>[2x]MSAQLRAAAAITPAARRVISGPAAVRRFHHYHHLPTGGIQRVEIAARGLRRSVQFPALANAYHNNAVIVRNASFTRLLPKLALKFIRVPALFGGMMLGAVGWVQYQAIKVSNSAQEFYGNIKATVADTAFSVWSSAVDIAEQTKRGWENTKNQFEIPEWLDRIMKGEGLAGEGSGSGEGGPNGGPEPPRQSRAGAATVAGASATVYGYGASDNDDRTPEEIMRDDNMMFITKKMIEIRNLLQKVGQGSTVTLPSIVVIG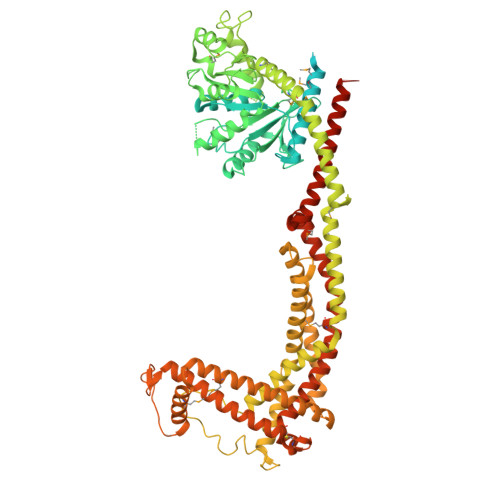SQSSGKSSVLEAIVGHEFLPKGSNMITRRPIELTLVNDPEAKVDYGEFPDLGLARVTDFSLIQKTLTELNQSVPESECVTDDPIRLTIHSPNIPDLSLIDLPGYIQVAGENQPRELKRKITELCDKYIRGPNIILAISAADTDLANSTALQASRRVDPRGERTIGVITKMDLVEPEKGAAILSDRQYPLKLGYVGVISKLPPQSGLFRRDTGNLLASINRNEKNYFGSHPTEFGPDSGVSTGVMTLRKKLLQVLEQQMSSKLNETTEAIQRELEETTYQFKVQYNEQPMSAESYLAASLDDFKHQFHEFASSFGRPQLQTLLKDALDQKVLDQLAARYWNRPIEDLSPAPREPDNIIDLPKADPDSPYWHRQLDTACSGLTRLGVGRLAATVAASAIQQHVEKLLDKSSFAKHPSARKVISDAAATVLADRSYATSDGIEISLKPYKFDPDIQPNEWAQGREHVVGVLQAELEQCQAAMKALENSVGGRKKLKEVMSFVDKARKGEIIVEGDHPSGAGGFSAALLARGREAVFLRDRADILSLRIQAAKSRQCKTLTNKYYCPEVFLDAVATKLAQTAVLFLNVEMLNDFYVRFPREVEAKLHEHMHAGGGLEKFAREDPKVRRHLDLIRRKELLETVLGKIEELHRISSGTAGTLGLRGAGDLKKRIGAPSSSGRRSFF>[2x]MKDYKSITIATEGSYAPYNFKDAGGKLIGFDIDLGNDLC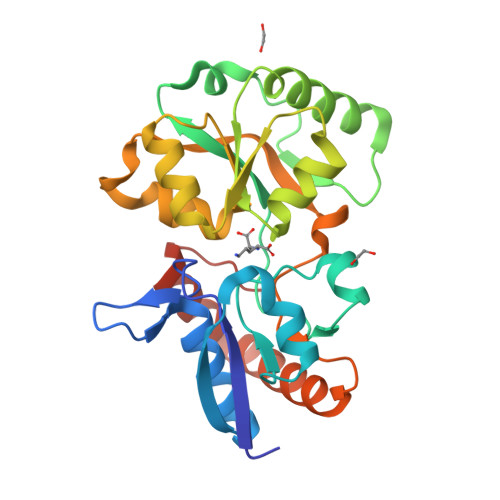KRMNIECKFVEQAWDGIIPSLTAGRYDAIMAAMGIQPAREKVIAFSRPYLLTPMTFLTTADSPLLKTQVAIENLPLDNITPEQKAELDKFTKIFEGVKFGVQAGTSHEAFMKQMMPSVQISTYDTIDNVVMDLKAGRIDASLASVSFLKPLTDKPDNKDLKMFGPRMTGGLFGKGVGVGIRKEDADLKALFDKAIDAAIADGTVQKLSQQWFGYDASPKQHHHHHH>[60x]MSLPPHQKVPLPSLSPTMQAGTIARWEKKEGDKINEGDLIAEVETDKATVGFESLEECYMAKILVAEGTRDVPIGAIICITVGKPEDIEAFKNYTLDSSAAPTPQAAPAPTPAATASPPTPSAQAPGSSYPPHMQVLLPALSPTMTMGTVQRWEKKVGEKLSEGDLLAEIETDKATIGFEVQEEGYLAKILVPEGTRDVPLGTPLCIIVEKEADISAFADYRPTEVTDLKPQVPPPTPPPVAAVPPTPQPLAPTPSAPCPATPAGPKGRVFVSPLAKKLAVEKGIDLTQVKGTGPDGRITKKDIDSFVPSKVAPAPAAVVPPTGPGMAPVPTGVFTDIPISNIRRVIAQRLMQSKQTIPHYYLSIDVNMGEVLLVRKELNKILEGRSKI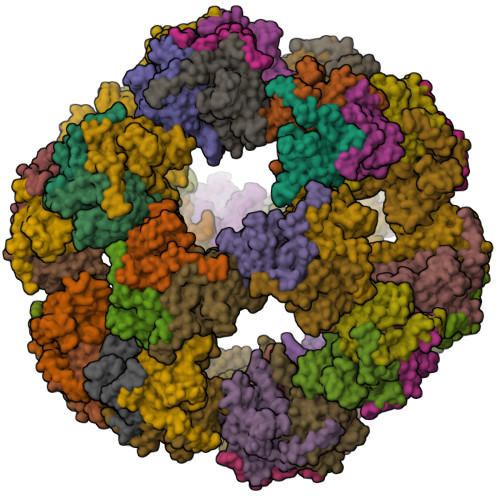SVNDFIIKASALACLKVPEANSSWMDTVIRQNHVVDVSVAVSTPAGLITPIVFNAHIKGVETIANDVVSLATKAREGKLQPHEFQGGTFTISNLGMFGIKNFSAIINPPQACILAIGASEDKLVPADNEKGFDVASMMSVTLSCDHRVVDGAVGAQWLAEFRKYLEKPITMLL>[2x]MRNDGGFLDWWEDLRSEMQSITDSQEVFAVLEKEVRRLGFDYYAYCVRHPIPFTRPRIFMFGNYPPAWQEHYQAQNYFAIDPTIRHCLRSGNHIVWSDDLFADAQELWDDARDYGLRHGATHSCMAPNGVMGFLSVARSSPAISPHEREELRLRMRCLIELLHQTLTELNHPSLQPQPICLSKREREILRWTADGKTSAEIAKILGISESTVNFHLKNIQKKFNAPNKTQAAAYAAALGLI

The majority of traits controlled by rhl transcription factor RhlR depend on PqsE, a dispensable thioesterase in Pseudomonas Quinolone Signal (PQS) biosynthesis that interferes with RhlR through an enigmatic mechanism likely involving direct interaction of both proteins. Here we show that PqsE and RhlR form a 2:2 protein complex that, together with RhlR agonist N-butanoyl-L-homoserine lactone (C4-HSL), solubilizes RhlR and thereby renders the otherwise insoluble transcription factor active. PqsE is a thioesterase that triggers transcription of the RhlR regulon through a hitherto cryptic mechanism, which we identify here as involving a significant chaperone-like component that enhances the stability of RhlR via protein complex formation. In common with many other gram-negative bacteria, two QS circuits use N-acyl-L-homoserine lactones (HSLs) as autoinducers, namely N-(3-oxododecanoyl)-L-HSL (3-oxo-C12-HSL) and N-butanoyl-L-HSL (C4-HSL), which are produced by autoinducer synthases LasI and RhlI and activate the LuxR-type transcription factors LasR and RhlR, respectively.

To corroborate this further, we sought to replace wildtype RhlR with an in-silico optimized variant that triggers pyocyanin production independently of PqsE and C4-HSL. Indeed, the PROSS-designed RhlR-P75, in which 75 (out of 241) residues were mutated with respect to the original sequence, could easily be produced in E. coli, even in the absence of C4-HSL or mBTL. The variant displayed a melting temperature of 84.3 ± 1.3 °C in the absence of ligands, which increased to over 90 °C in buffer containing 1 mM mBTL, nearly 40 K higher than the WT protein under similar conditions. It crystallized readily in the presence of C4-HSL or mBTL, but not without these ligands. A complex with mBTL diffracted to 2.15 Å resolution and yielded well-resolved electron density for the ligand. The butanol-m-bromophenol group of mBTL resides in the hydrophobic acyl-binding tunnel leading towards the lactone binding site, and the m-bromophenol establishes π-stacking interactions with Y64 and Y72, two residues also contained in wildtype RhlR. Co-expression of RhlR-P75 and His6-tagged PqsE revealed that the interaction between both proteins has been lost by the introduced mutations.4,6-dideoxy-4-{[(1S,4R,5S,6S)-4,5,6-trihydroxy-3-(hydroxymethyl)cyclohex-2-en-1-yl]amino}-alpha-D-glucopyranose | C13 H23 N O8 | 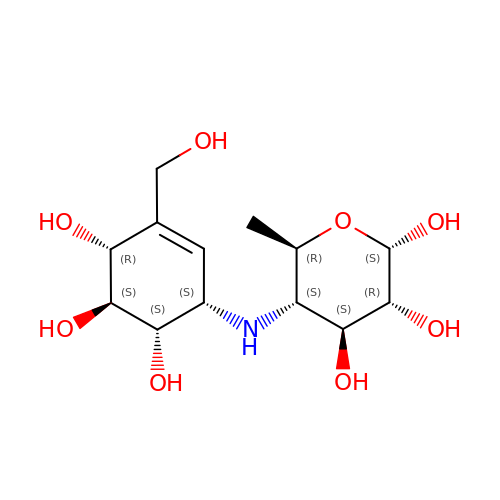RBZIIHWPZWOIDU-ZCGMLSCUSA-N> MRNQELARIFEEIGLMSEFLGDNPFRVRAYHQAARTLYDLDTPIEEIAEKGKEALMELPGVGPDLAEKILEFLRTGKVRKHEELSRKVPRGVLEVMEVPGVGPKTARLLYEGLGIDSLEKLKAALDRGDLTRLKGFGPKRAERIREGLALA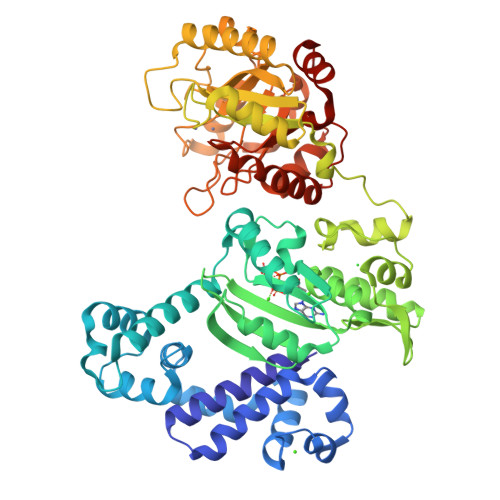QAAGKRRPLGAVLSLARSLLEAIRALPGVERAELCGSARRYKDTVGDLDFLVASREGERAVEGFVRLPQVKEVYAKGKERATVFLKNGLQVDLRVVPPESYGAGLQYLTGSAAHSIRLRALAQEKGLKLSEYGVFRGEKRIAGETEEEVYAALGLPWIPPPLREDQGEVEAALEGRLPKLLELPQVKGDLQVHSTYSDGQNTLEELWEAAKTMGYRYLAVTDHSPAVRVAGGPSPEEALKRVGEIRRFNETHGPPYLLAGAEVDIHPDGTLDYPDWVLRELDLVLVSVHSRFNLPKADQTKRLLKALENPFVHVLAHPTARLLGRRAPIEADWEAVFQKAKEKGVAVEIDGYYDRMDLPDDLARMAYGMGLWISLSTDAHQTDHLRFMELAVGTAQRAWIGPERVLNTLDYEDLLSWLKARRGV> MFRAAAPGQLRRAASLLRFQSTLVIAEHANDSLAPITLNTITAATRLGGEVSCLVAGTKCDKVAQDLCKVAGIAKVLVAQHDVYKGLLPEELTPLILATQKQFNYTHICAGASAFGKNLLPRVAAKLEVAPISDIIAIKSPDTFVRTIYAGNALCTVKCDEKVKVFSVRGTSFDAAATSGGSASSEKASSTSPVEISEWLDQKLTKSDRPELTGAKVVVSGGRGLKSGENFKLLYDLADQLHAAVG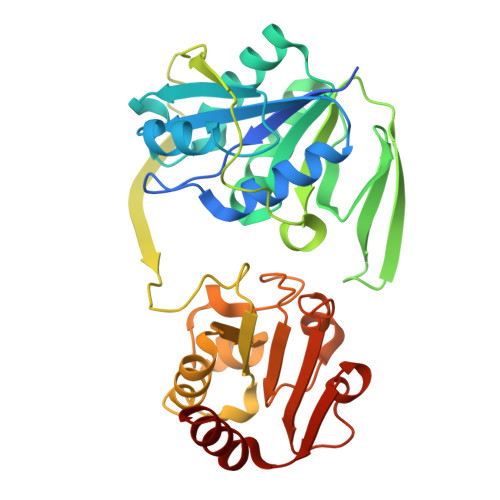ASRAAVDAGFVPNDMQVGQTGKIVAPELYIAVGISGAIQHLAGMKDSKTIVAINKDPEAPIFQVADYGIVADLFKVVPEMTEILKKK(2R)-2-{[(2S)-2-(4-cyanophenyl)propyl]amino}-N-[5-(1-methyl-1H-pyrazol-4-yl)pyridin-2-yl]-2-phenylacetamide 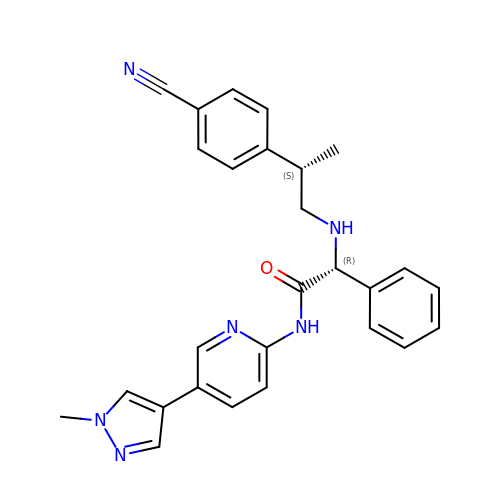| C27 H26 N6 O | SEDFZSHSBUXKAC-NIYFSFCBSA-N> IAPITGTIKRRVIMDIVLGFSLGGVMASYWWWGFHMD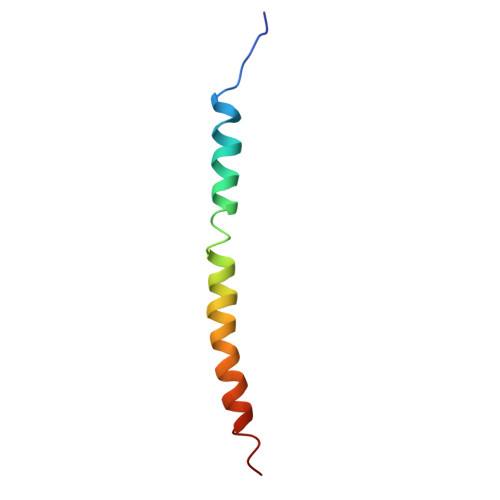KINKREKFYAELAERK>[2x]MGSITENTSWNKEFSAEAVNGVFVLCKSSSKSCA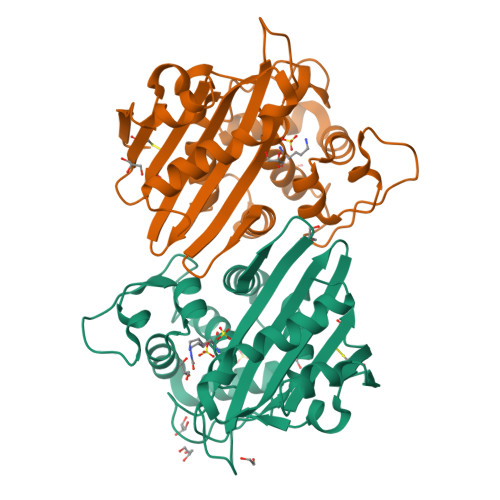TNDLARASKEYLPASTFKIPNAIIGLETGVIKNEHQVFKWDGKPRAMKQWERDLTLRGAIQVSAVPVFQQIAREVGEVRMQKYLKKFSYGNQNISGGIDKFHLEGQLRISAVNQVEFLESLYLNKLSASKENQLIVKEALVTEAAPEYLVHSKTGFSGVGTESNPGVAWWVGWVEKETEVYFFAFNMDIDNESKLPLRKSIPTKIMESEGIIGG> GSDVVDPDIFNRDPRDHYDLLQRLGGGTYGEVFKARDKVSGDLVALKMVKMEPDDDVSTLQKEILILKTCRHANIVAYHGSYL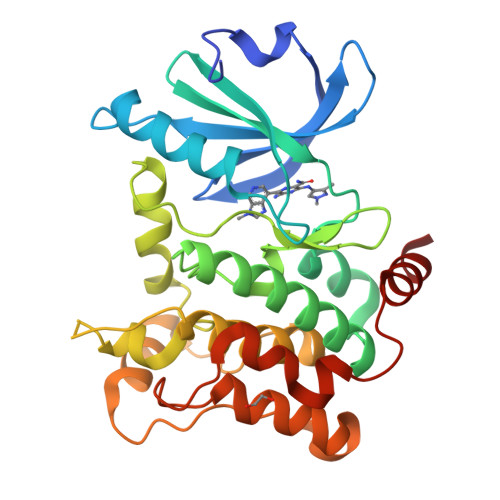WLQKLWICMEFCGAGSLQDIYQVTGSLSELQISYVCREVLQGLAYLHSQKKIHRDIKGANILINDAGEVRLADFGISAQIGAELARRLEFIGTPYWMAPEVAAVALKGGYNELCDIWSLGITAIELAELQPPLFDVHPLRVLFLMTKSGYQPPRLKEKGKWSAAFHNFIKVTLTKSPKKRPSATKMLSHQLVSQPGLNRGLILDLLDKLKN Hyperpolarization and cyclic nucleotide (HCN) activated ion channels are critical for the automaticity of action potentials in pacemaking and rhythmic electrical circuits in the human body. Unlike most voltage-gated ion channels, the HCN and related plant ion channels activate upon membrane hyperpolarization. HCN channels are also regulated by cyclic nucleotides, which act via the CNBD and fine-tune the frequency of their pacemaking activity. Here, we present cryo-electron microscopy structures of human HCN1 corresponding to Closed, Open, and a putative Intermediate state.

We found that HCN1-F186C-S264C mutant in a mixture of 0.0025% LMNG, soy polar lipids, and cholesterol hemi-succinate elutes primarily as a monodisperse peak. This fraction was collected, and its structure was determined in the presence of Hg2+ to a global resolution of 3.6 Å using single-particle cryo-EM. Thus, we conclude that the Open channel conformation is primarily facilitated by oxidizing conditions that trap the voltage sensors in a hyperpolarized conformation. In the Open state, the R4 charge moves past this position by a complete helical turn and the S4 helix retains its mid-helical bend in the Open state. Another unique feature is that the intracellular end of the S4 helix unwinds and shortens by about two helical turns in the Open-state structure. However, the diameter of the pore gate in the Open structure increases significantly to about 7.4 Å, driven by the dilation of the S6 helices and rotation of the residues Y386, T394, and Q398 away from the pore axis. Notably, the selectivity filter in the Open state undergoes conformational rearrangement simultaneously with gating transitions at the pore gates, leading to pore expansion in the selectivity filter. Upon further examination of the cryo-EM densities, we discovered that C309 in the S5 helix and C385 in S6 likely form a disulfide bridge in the Open but not in the Closed state. Concomitant with these structural changes in the S4 and S5 helices, the residues in this region make extensive contact with the B’ helix of the C-linker region in the Open state. All-atom simulations of ion permeation through the Open-state structure in a lipid bilayer with an applied voltage clearly show that this channel pore is conducting.

>MEGGGKPNSSSNSRDDGNSVFPAKASATGAGPAAAEKRLGTPPGGGGAGAKEHGNSVCFKVDGGGGGGGGGGGGEEPAGGFEDAEGPRRQYGFMQRQFTSMLQPGVNKFSLRMFGSQKAVEKEQERVKTAGFWIIHPYSDFRFYWDLIMLIMMVGNLVIIPVGITFFTEQTTTPWIIFNVASDTVCLLDLIMNFRTGTVNEDSSEIILDPKVIKMNYLKSWFVVDFISSIPVDYIFLIVEKGMDSEVYKTARALRIVRFTKILCLLRLLRLSRLIRYIHQWEEIFHMTYDLASAVVRIFNLIGMMLLLCHWDGCLQFLVPLLQDFPPDCWVSLNEMVNDSWGKQYSYALFKAMSHMLCIGYGAQAPVSMSDLWITMLSMIVGATCYAMFVGHATALIQSLDSSRRQYQEKYKQVEQYMSFHKLPADMRQKIHDYYEHRYQGKIFDEENILNELNDPLREEIVNFNCRKLVATMPLFANADPNFVTAMLSKLRFEVFQPGDYIIREGAVGKKMYFIQHGVAGVITKSSKEMKLTDGSYFGEICLLTKGRRTASVRADTYCRLYSLSVDNFNEVLEEYPMMRRAFETVAIDRLDRIGKKNSILLQKFQKDLNTGVFNNQENEILKQIVKHDREMVQAIAPINYPQMTTLNSTSSTTTPTSRMRTQSPPVYTATSLSHSNLHSPSPSTQTPQPSAILSPCSYTTAVCSPPVQSPLAARTFHYASPTASQLSLMQQQPQQQVQQSQPPQTQPQQPSPQPQTPGSSTPKNEVHKSTQALHNTNLTREVRPLSASQPSLPHEVSTLISRPHPTVGESLASIPQPVTAVPGTGLQAGGRSTVPQRVTLFRQMSSGAIPPNRGVPPAPPPPAAALPRESSSVLNTDPDAEKPRFASNL[4x]>[14x]MGQAFFKKIVGCFCLGYLFLSSAIEAAALDIKNFNRGRVKVVNKKIAYLGDEKPITIWTSLDNVTVIQLEKDETISYITTGFNKGWSIVPNSNHIFIQPKSVKSNLMFEKEAVNFALMTRDYQEFLKTKKLIVDAPDPKELEEQKKALEKEKEAKEQAQKAQKDKREKRKEERAKNRANLENLTNAMSNPQNLSNNKNLSEFIKQQRENELDQMERLEDMQEQAQANALKQIEELNKKQAEETIKQRAKDKINIKTDKPQKSPEDNSIELSPSDSAWRTNLVVRTNKALYQFILRIAQKDNFASAYLTVKLEYPQRHEVSSVIEEELKKREEAKRQK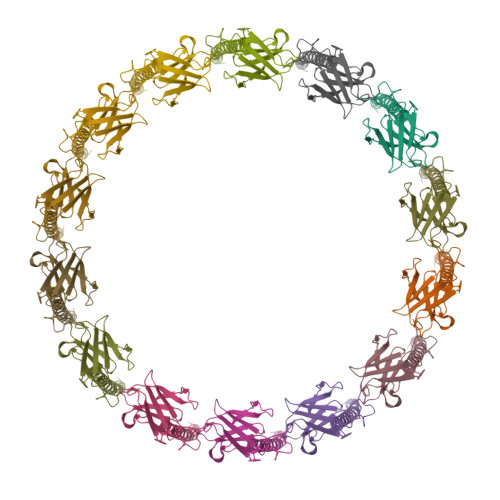ELIKQENLNTTAYINRVMMASNEQIINKEKIREEKQKIILDQAKALETQYVHNALKRNPVPRNYNYYQAPEKRSKHIMPSEIFDDGTFTYFGFKNITLQPAIFVVQPDGKLSMTDAAIDPNMTNSGLRWYRVNEIAEKFKLIKDKALVTVINKGYGKNPLTKNYNIKNYGELERVIKKLPLVRDK>SHMTTSIDPTTPLTYNPVIDALVGSWRQIIDADYSADDTRLPDLAVLARSTARAVAAAVPRPLAEISAPDAPDERGELVLLEKVIQEVADREYTPLSPEGPSVGDLVLVTEKIYNSDREEIGADTGRLRIIRKDPETGHHFTVSLVTSTVQGNKLFAFGYTEMEAQLAGG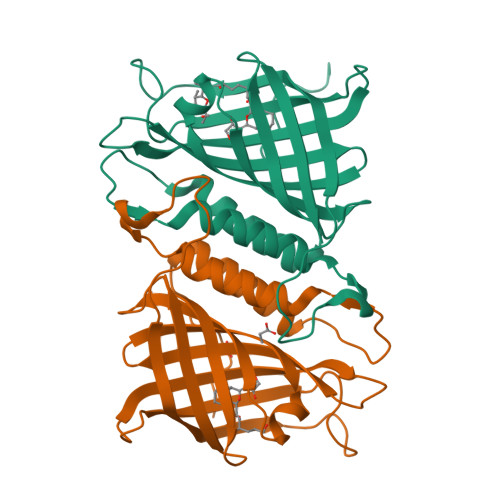RTTIQVACWDGPWAGMSGTLSWVINSMTAAESRYELRR[2x]> MDFLDFEKVFSFYSKATKKGFSPFFVPALEKAEEPAGNFFLDRKGNLFSIREDFTKTVLNHRKRYSPDSQIKVWYADFVYRYSGSDLVAEYQLGLEKVPRNSLDDSLEVLEIIVESASEFFEGP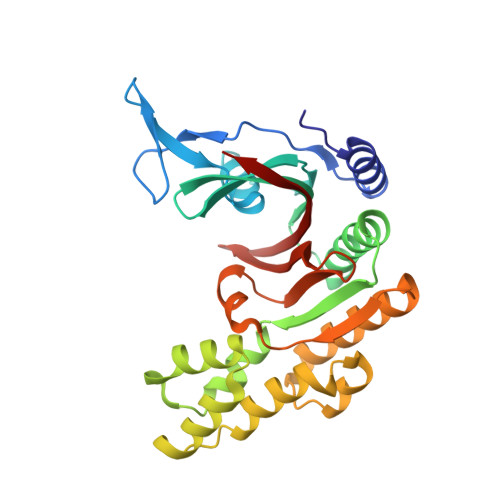VIVEIGHTGVYEDLLKEIPKDLHEKVLNLIDTKNLAEIEFLSHMKKIDLSRVEKIIEDSIYRRSPEHLKTMDLPLSVREDLLSASSFLQEKFPTVSVEIDLTLARTIEEYCGLIFTIYDTSSSRLVAAGGEYTVNGEKGVGGSIFLEGKTC> SNAMTIKGRAFPEGFLWGGAVAAHQLEGGYKEGGKGLSTADIMTLGTNERPREITDGVVAGKYYPNHQAIDFYHRYPEDIELFAEMGFKCFRTSIAWTRIFPNGDESEPNEAGLQFYDDLFDECLKNGIQPVVTLAHFEMPYHLVKQYGGWRNRKLIQFYLNFAKVCFERYRDKVTYWMTFNEINNQTNFESDGAMLTDSGIIHQPGENRERWMYQAAHYELVASAAAVQLGHQINPDFQIGCMIAMCPIYPLTAAPADVLFAQRAMQTRFYFADVHCNGTYPQWLRNRFESEHFNLDITAEDLKILQAGTVDYIGFSYYMSFTVKDTGKLAYNEEHDLVKNPYVKASDWGWQVDPVGLRYAMNWFTDRYHLPLFIVENGLGAIDKKTADNQIHDDYRIDYLTDHLRQIKLAVLEDGVDLIGYTPWGCIDLVAASTGQMSKRYGFIYVDENDDGSGSLKRYKKDSFTWFQHVIATNGAEIE

Specifically, the β-­glycosidic bond of 6′-P-β-glucoside is cleaved by 6-P-β-glucosidase (6PβGlu; EC 3.2.1.86), releasing 6-P-β-glucose (BG6; glycon), an important cellular precursor, and the remaining portion of the given substrate (aglycon). Here, the high-resolution crystal structures of GH1 6-P-β-glucosidases from Lactobacillus plantarum (LpPbg1) and Streptococcus mutans (SmBgl) and their complexes with ligands are reported. 6PβGlu is a single-domain protein that adopts a (β/α)8-barrel (TIM-barrel) structure, which is a typical fold of GH1-family members. The GH1-family enzymes utilize a double-displacement mechanism of catalysis with retention of configuration at the anomeric C atom of the glycon moiety.

The LpPbg1 structure has been determined in an apo form as well as in a complex with phosphate and a glucose molecule corresponding to the aglycon molecule. The final model also included 590 water molecules, four phosphate anions, one acetate anion and one glucose molecule. In LpPgb1, the phosphate moiety interacts with the side chains of Lys438, Tyr440 and Ser432. Additional anchoring points are provided by the main-chain amides of Ala431 and Ser432. The ligand was most likely acquired during cryoprotection with sucrose solution (1.55 M) that must also have contained some glucose. Since the phosphate binding site was already occupied by a phosphate ion, soaked glucose could not be accommodated in the −1 subsite because the sugar O6 hydroxyl group would clash with the anion moiety. Therefore, it was bound in the aglycon-dedicated portion of the active site. The molecule interacts directly via hydrogen bonds linking O2 and O3 to the guanidinium group of Arg267 and O3 to Asn183. In contrast to other enzymes, LpPgb1 binds its aglycon ligand very tightly through numerous hydrogen bonds. As LpPgb1 possesses similar activity, it is likely that the glucose-binding mode in the +1 subsite mimics the binding of the aglycon moiety of 6-P-gentiobiose that contains the β-(1→6)-glycosidic bond.> HHHHHHHSEMTPREIVSELDKHIIGQDNAKRSVAIALRNRWRRMQLNEELRHEVTPKNILMIGPTGVGKTEIARRLAKLANAPFIKVEATKFTEVGYVGKEVDSIIRDLTDAAVKMVRVQAIEKNRYRAEELAEERILDVLIPPAKNNWGQTEQQQEPSAARQAFRKKLREGQLDDKEIEIDLAAAPMGVEIMAPPGMEEMTSQLQSMFQNLGGQKQKARKLKIKDAMKLLIEEEAAKLVNPEELKQDAIDAVEQHGIVFIDEIDKICKRGESSGPDVSREGVQRDLLPLVEGCTVSTKHGMVKTDHILFIASGAFQIAKPSDLIPELQGRLPIRVELQALTTSDFERILTEPNASITVQYKALMATEGVNIEFTDSGIKRIAEAAWQVNESTENIGARRLHTVLERLMEEISYDASD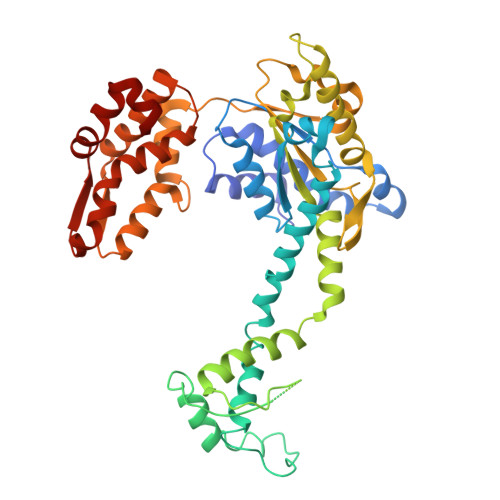LSGQNITIDADYVSKHLDALVADEDLSRFIL> MLDPGEVYDDPIDPIELEAEPRGTPIVPNILRNSDYNLNSPLIEDPARLMLEWLKTGNRPYRMTLTDNCSRSFRVLKDYFKKVDLGSLKVGGMAAQSMISLWLYGAHSESNRSRRCITDLAHFYSKSSPIEKLLNLTLGNRGLRIPPEGVLSCLERVDYDNAFGRYLANTYSSYLFFHVITLYMNALDWDEEKTILALWKDLTSVDIGKDLVKFKDQIWGLLIVTKDFVYSQSSNCLFDRNYTLMLKDLFLSRFNSLMVLLSPPEPRYSDDLISQLCQLYIAGDQVLSMCGNSGYEVIKILEPYVVNSLVQRAEKFRPLIHSLGDFPVFIKDKVSQLEETFGPCARRFFRAL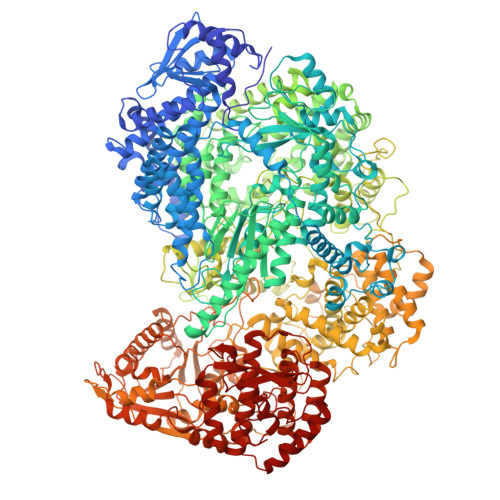DQFDNIHDLVFVFGCYRHWGHPYIDYRKGLSKLYDQVHLKKMIDKSYQECLASDLARRILRWGFDKYSKWYLDSRFLARDHPLTPYIKTQTWPPKHIVDLVGDTWHKLPITQIFEIPESMDPSEILDDKSHSFTRTRLASWLSENRGGPVPSEKVIITALSKPPVNPREFLRSIDLGGLPDEDLIIGLKPKERELKIEGRFFALMSWNLRLYFVITEKLLANYILPLFDALTMTDNLNKVFKKLIDRVTGQGLLDYSRVTYAFHLDYEKWNNHQRLESTEDVFSVLDQVFGLKRVFSRTHEFFQKAWIYYSDRSDLIGLREDQIYCLDASNGPTCWNGQDGGLEGLRQKGWSLVSLLMIDRESQIRNTRTKILAQGDNQVLCPTYMLSPGLSQEGLLYELERISRNALSIYRAVEEGASKLGLIIKKEETMCSYDFLIYGKTPLFRGNILVPESKRWARVSCVSNDQIVNLANIMSTVSTNALTVAQHSQSLIKPMRDFLLMSVQAVFHYLLFSPILKGRVYKILSAEGESFLLAMSRIIYLDPSLGGISGMSLGRFHIRQFSDPVSEGLSFWREIWLSSQESWIHALCQEAGNPDLGERTLESFTRLLEDPTTLNIRGGASPTILLKDAIRKALYDEVDKVENSEFREAILLSKTHRDNFILFLISVEPLFPRFLSELFSSSFLGIPESIIGLIQNSRTIRRQFRKSLSKTLEESFYNSEIHGISRMTQTPQRVGGVWPCSSERADLLREISWGRKVVGTTVPHPSEMLGLLPKSSISCTCGATGGGNPRVSVSVLPSFDQSFFSRGPLKGYLGSSTSMSTQLFHAWEKVTNVHVVKRALSLKESINWFITRDSNLAQALIRNIMSLTGPDFPLEEAPVFKRTGSALHRFKSARYSEGGYSSVCPNLLSHISVSTDTMSDLTQDGKNYDFMFQPLMLYAQTWTSELVQRDTRLRDSTFHWHLRCNRCVRPIDDVTLETSQIFEFPDVSKRISRMVSGAVPHFQRLPDIRLRPGDFESLSGREKSHHIGSAQGLLYSILVAIHDSGYNDGTIFPVNIYGKVSPRDYLRGLARGVLIGSSICFLTRMTNININRPLELVSGVISYILLRLDNHPSLYIMLREPSLRGEIFSIPQKIPAAYPTTMKEGNRSILCYLQHVLRYEREIITASPENDWLWIFSDFRSAKMTYLSLITYQSHLLLQRVERNLSKSMRDNLRQLSSLMRQVLGGHGEDTLESDDNIQRLLKDSLRRTRWVDQEVRHAARTMTGDYSPNKKVSRKVGCSEWVCSAQQVAVSTSANPAPVSELDIRALSKRFQNPLISGLRVVQWATGAHYKLKPILDDLNVFPSLCLVVGDGSGGISRAVLNMFPDAKLVFNSLLEVNDLMASGTHPLPPSAIMRGGNDIVSRVIDLDSIWEKPSDLRNLATWKYFQSVQKQVNMSYDLIICDAEVTDIASINRITLLMSDFALSIDGPLYLVFKTYGTMLVNPNYKAIQHLSRAFPSVTGFITQVTSSFSSELYLRFSKRGKFFRDAEYLTSSTLREMSLVLFNCSSPKSEMQRARSLNYQDLVRGFPEEIISNPYNEMIITLIDSDVESFLVHKMVDDLELQRGTLSKVAIIIAIMIVFSNRVFNVSKPLTDPSFYPPSDPKILRHFNICCSTMMYLSTALGDVPSFARLHDLYNRPITYYFRKQVIRGNVYLSWSWSNDTSVFKRVACNSSLSLSSHWIRLIYKIVKTTRLVGSIKDLSREVERHLHRYNRWITLEDIRSRSSLLDYSCL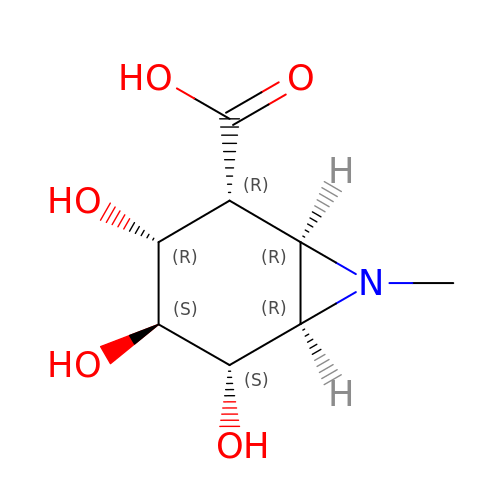(1~{R},2~{R},3~{R},4~{S},5~{S},6~{R})-7-methyl-3,4,5-tris(oxidanyl)-7-azabicyclo[4.1.0]heptane-2-carboxylic acid | C8 H13 N O5 | UUIBNQLYUYNUOZ-FKAYCGLJSA-N> NT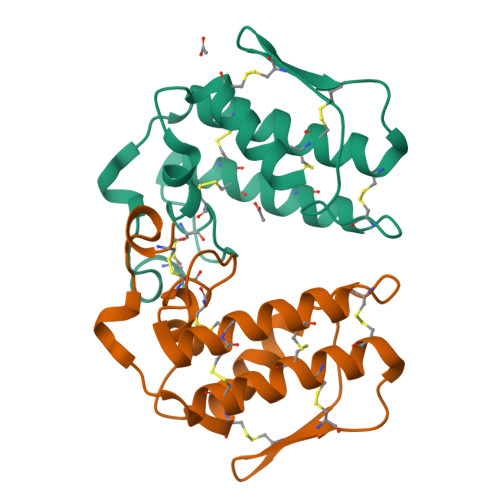YQFKNMIQCTVPKRSWWDFADYGCYCGRGGSGTPIDDLDRCCQVHDNCYNSAREQGGCRPKQKTYSYECKAGTLSCSGSNNSCAATVCDCDRLAAICFAGAPYNDNNYNIDLKARCQ;> NRWQFKNMISCTVPSRSWWDFADYGCYCGRGGSGTPVDDLDRCCQVHDNCYNEAEKISGCNPRFRTYSYECTAGTLTCTGRNNACAASVCDCDRLAAICFAGAPYNDNNYNIDLQARCN>[4x]MSTEKFTITEHLVPGSHIREYPGSTVNQEDVLKIHVKQYTPKREGPVPDDAITFIATHGVGLPKELYEPLWDELLDQASGFHIRAIWMADVASMNQSGIHNEDKLSMDCSWMDHARDLLLMINHFRDQMPRP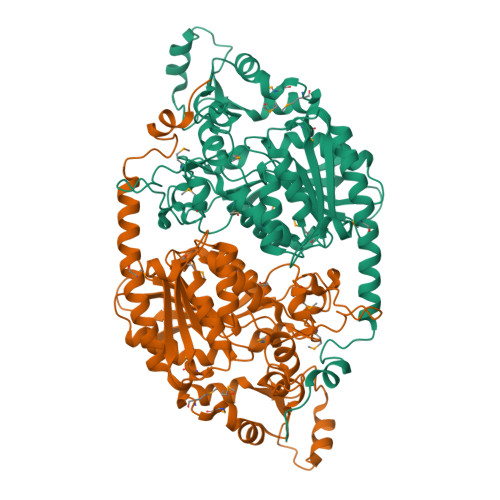LVGIGHSFGGNIITNLAYLHPRLFTTLLLLDPLIQLSPPSLGFGTDAPSAINYTLWRDDVWPSREVAIRANRAIMQGMDPRCLDRMTKHFFRDLPTPLYPDVEAIKALFGTTADSTTTPVTLTTPKYHELVAQIRQNFNARDPKTGRIEVPRDTHADMDPLVAYIPLYRPEPRSTFRRLETLRPSCLWVIAGATFLNIDEIREGVKICGSGIGGSGGVPDGRVREVVLPGFGHLMPFQEVKTVAETCIVWLQQEMDRFRQTERQWKEDRDGKSHLAVEENWYKVLKPIPSGRKKRNDKGKL> MALNRVPSRVLPFAVSGVYVHPRNACRLPAAAAVSSVPSSVSAFSSRTNFLSRSSSAVMSHPCAATARHFSFAIPPANAAALADPLPATPTPPPVFEAVSSASSGIASGTNALKNVEEVSTMERYEAAVYEESFKKPIVCLFFARFSLQSKVLLQPFLDFA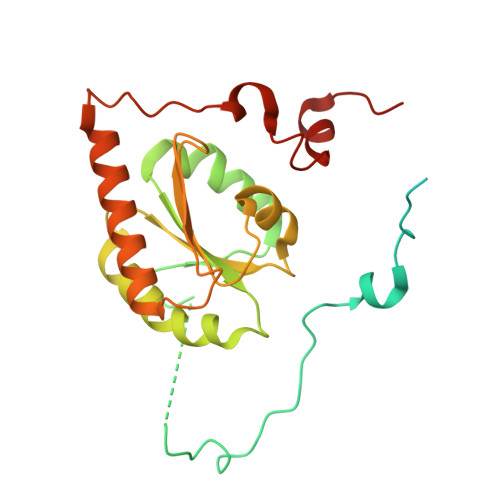ASASNNATFFLIDCDRVPRAAYHARVENVPSLVVMKGDDAFRQTITDSVGVKTAGDLIQEARSALDQVLRLDQQEGGTKLQPGVSSYTHHIGVDNLNVYRKGWPVA>[4x]GSYDSSSSSSNDSSARNEEDESCMFALKLLGGFAVPFTIKAVIELGVMDQLLTAERAMSAEELVAAAVAAQLPRPEVACTMVDRLLRFLASHSVVRCTTEVVVGTDDATTTTCCRRSYAASPVCKWFARNGVEDSVLPLGMMILNKTFLDSWQNITDAVLEGAAPFEKTYGMPMFEYLSTNGPLNTVFHEAMANHSMIITKKLLKFFRGFEGLDVLVDVGGGNGTTLQMIRGQYKNMRGINYDLPHVIAQAAPVEGVEHVGGSMFDNIPRGNAVLLKWILHDWDDKACIKILKNCYTALHVRGKVIVLEYVVPDEPEPTLAAQGAFELDLTMLVTFGSGKERTQREFSELAMEAGFSREFKATYIFANVWALEFTK

A stilbene O-methyltransferase, SbSOMT, is first shown to be indispensable for pathogen-inducible pterostilbene (3,5-bis-O-methylated) biosynthesis in sorghum (Sorghum bicolor). Phylogenetic analysis indicates the recruitment of genus-specific SOMTs from canonical caffeic acid O-methyltransferases (COMTs) after the divergence of Sorghum spp. from Saccharum spp. In recombinant enzyme assays, SbSOMT and COMTs regioselectively catalyze O-methylation of stilbene A-ring and B-ring respectively. Whilst SbSOMT shows global structural resemblance to SbCOMT, molecular characterizations illustrate two hydrophobic residues (Ile144/Phe337) crucial for substrate binding orientation leading to 3,5-bis-O-methylations in the A-ring. The catalytic residues of SbSOMT are highly conserved with all reported COMTs, including His282 as the key nucleophile, whereas Asp283, Glu310, and Glu342 collectively charge the basicity or confine His282 in its reactive conformation.

To rationalize their different catalytic regioselectivities, structural analyses involving X-ray crystallography and computational methods were conducted. We solved the crystal structure of an SbSOMT-resveratrol-nicotinamide adenine dinucleotide (β-NAD) ternary complex (diffracted to 1.72 Å resolution, Fig. 4d; β-NAD was utilized as an additive to improve crystallization), an SbSOMT-resveratrol binary complex, and two ternary complexes reproduced with pinostilbene or pterostilbene (diffracted at 2.10 and 2.56 Å, respectively). All complexes were in high structural resemblance and depicted as a homodimer with an open conformation. Of the three hydroxyl groups on resveratrol capable of forming hydrogen bonds, only the methyl-accepting 3-OH group (A-ring) formed direct hydrogen bonds to SbSOMT residues, including the catalytic residues His282 (2.80 Å) and Asp283 (3.26 Å). Other hydroxyl groups were shielded by water molecules and did not directly interact with SbSOMT. Overall, these structures depicted a productive substrate orientation within the substrate binding pocket which greatly favors A-ring O-methylation. So far, our results revealed that SbSOMT catalyzes the 3,5-bis-O-methylation of resveratrol upon fungal infection.>[4x]IVGGSDAKEGAWPWVVGLYYDD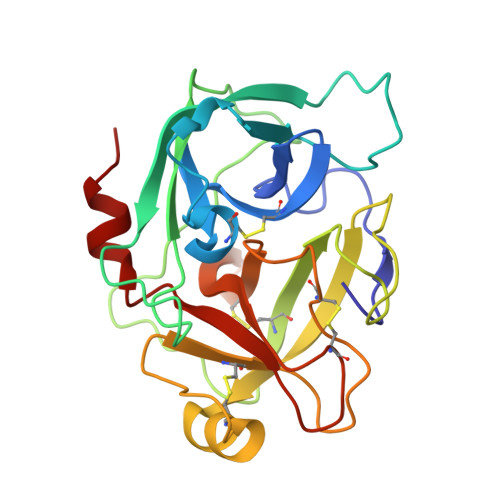RLLCGASLVSSDWLVSAAHCVYGRNLEPSKWTAILGLHMKSNLTSPQTVPRLIDEIVINPHYNRRRKDNDIAMMHLEFKVNYTDYIQPISLPEENQVFPPGRNCSIAGWGTVVYQGTTADILQEADVPLLSNERCQQQMPEYNITENMICAGYEEGGIDSCQGDSGGPLMCQENNRWFLAGVTSFGYECALPNRPGVYARVSRFTEWIQSFLH>[2x]CPGGCSCDHIPGSGLKMNCNNRNVSSLADLKPKLSNVQELFLRDNKIHSIRKSHFVDYKNLILLDLGNNNIATVENNTFKNLLDLRWLYMDSNYLDTLSREKFAGL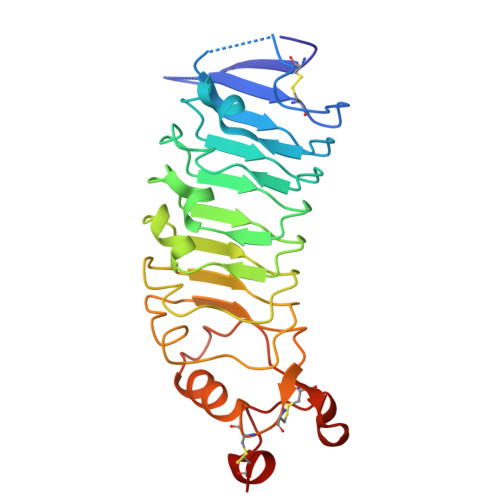QNLEYLNVEYNAIQLILPGTFNAMPKLRILILNNNLLRSLPVDVFAGVSLSKLSLHNNYFMYLPVAGVLDQLTSIIQIDLHGNPWECSCTIVPFKQWAERLGSEVLMSDLKCETPVNFFRKDFMLLSNDEICPQ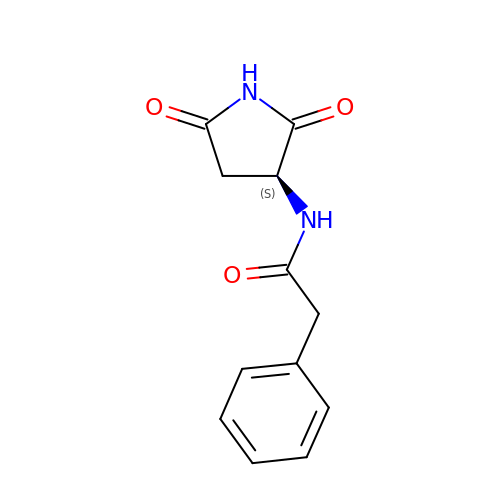~{N}-[(3~{S})-2,5-bis(oxidanylidene)pyrrolidin-3-yl]-2-phenyl-ethanamide | C12 H12 N2 O3 | ZTMDMWMWWGOUHX-VIFPVBQESA-N>GLGGMSVNTGEVFCSVPGRLSLLSSTSKYKVTVGEVQRRLSPPECLNASLLGGVLRRAKSKNGGRSLRERLEKIGLNLPAGRRKAANVTLLTSLVEGEAVHLARDFGYICETEFPAKAVSEYLNRQHTDPSDLHSRKNMLLATKQLCKEFTDLLAQDRTPIGNSRPSPILEPGIQSCLTHFSLITHGFGAPAICAALTALQNYLTEAL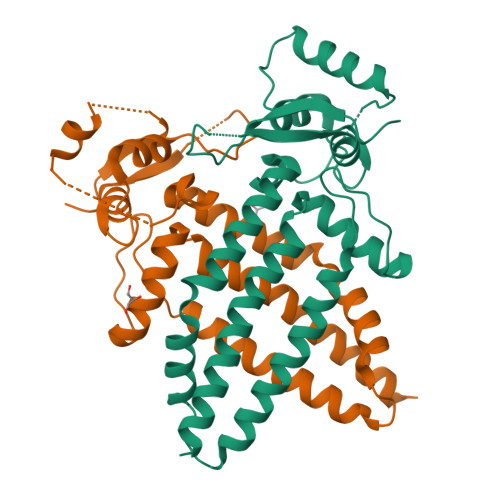KGMDKMFLNNTTTNRHTSGEGPGSKTGDKEEK[2x]>[2x]GDLVKPDAFSVKIQDWGSTEYDVTLNLGGTYDWVVKVK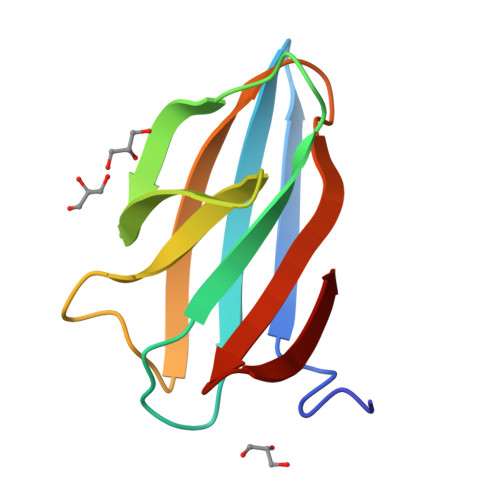LKDGSAVSSVWSANKAEEGGYVVFTPVSWNKGPTATFGFIATGSEPVEAMYLYVNDQLWDVW Ribonucleotide reductases (RNRs) catalyze the conversion of ribonucleotides to deoxyribonucleotides, a conserved reaction that is fundamental to DNA-based life. Nearly all aerobic organisms use class I RNRs, which consist of two subunits: α, which contains the catalytic site, and β, which houses a subclass-dependent metal center. Contrary to all other class Ib RNRs studied to-date, the sole RNR of Bacillus subtilis displays class Ia-like activity regulation. We find that B. subtilis RNR has arrived at a remarkably similar solution to the ATP-cone through the evolution of two unique allosteric sites that modulate catalytic activity by inducing contrasting quaternary interactions that either enable or prevent the full range of motions needed for RNR activity.

With insight from SAXS (see the section “Methods”), a 2.50 Å resolution crystal structure of the S-dimer was obtained by co-crystallizing holo-NrdE with 5 mM Mg2+-ATP, 0.5 mM TTP, and 1 mM GDP. Electron density at the S-site could be unambiguously modeled as TTP coordinating a Mg2+ ion. Electron density at the I-site showed strong evidence for an ADP ligand displacing dAMP. As ADP was not present in the crystallization condition, we suspect that it is a hydrolysis product of ATP (see the section “Methods”). Interestingly, we also observed nearby electron density for an ATP ligand with the adenine ring positioned against the F47-loop. Regardless, an important consequence of either ATP or GDP bound to the F47-loop is that the F47 side-chain flips inward by ~90° to form a π-stacking interaction with the purine ring. With F47 in this conformation, it is unable to participate in the formation of an I-dimer interface. Unexpectedly, we were able to trap the final six residues of the NrdE C-terminus in the catalytic site of our 2.50 Å structure due to partial disulfide formation between the tail cysteines (C695, C698) and two catalytic-site cysteines (C382, C170). These linkages, particularly that involving C695 and the initial site of the catalytically essential thiyl radical, C382, are likely artifacts of sample oxidation. However, they allowed us to capture the flexible C-terminus, which has never before been visualized in any class I RNR.

> MSQNQVPKWIQLNNEIMIQKDGKFQFDKDKEAVHSYFVDYINQNTVFFHNLKEKLDYLVENQYYEEEFLSLYSFEDIKEVFKTAYAKKFRFPSFMSAFKFYNDYALKTNDKKKILERYEDRISIVALFFANGDTEKAKEYVNLMINQEYQPSTPTFLNAGRKRRGELVSCFLLEVNDSLNDISRAIDISMQLSKLGGGVSLNLSKLRAKGEAIKDVENATKGVVGVMKLLDNAFRYADQMGQRQGSGAAYLNIFHRDINDFLDTKKISADEDVRVKTLSIGVVIPDKFVELAREDKAAYVFYPHTIYKEYGQHMDEMDMNEMYDKFVDNPRVKKEKINPRKLLEKLAMLRSESGYPYIMFQDNVNKVHANNHISKVKFSNLCSEVLQASQVSSYTDYDEEDEIGLDISCNLGSLNILNVMEHKSIEKTVKLATDSLTHVSETTDIRNAPAVRRANKAMKSIGLGAMNLHGYLAQNGIAYESPEARDFANTFFMMVNFYSIQRSAEIAKEKGETFDQYEGSTYATGEYFDKYVSTDFSPKYEKIANLFEGMHIPTTEDWKKLKAFVAEHGMYHSYRLCIAPTGSISYVQSSTASVMPIMERIEERTYGNSKTYYPMPGLASNNWFFYKEAYDMDMFKVVDMIATIQQHIDQGISFTLFLKDTMTTRDLNRIDLYAHHRGIKTIYYARTKDTGQDSCLSCVV> MESKRNKPGKA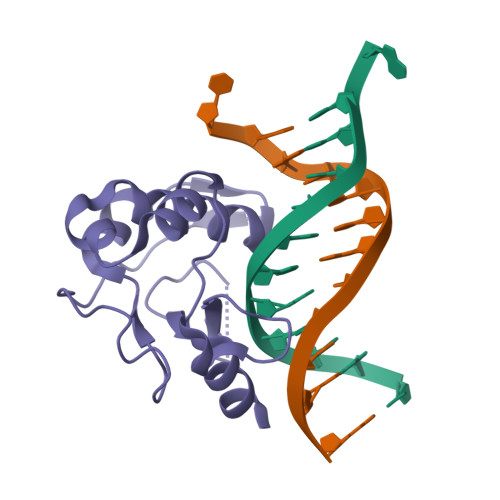TGKGKPVNNKWLNNAGKDLGSPVPDRIANKLRDKEFKSFDDFRKKFWEEVSKDPELSKQFSRNNNDRMKVGKAPKTRTQDVSGKRTSFELHEEKPISQNGGVYDMDNISVVTPKRHIDIHRGK> DLGSSQNVNVSSLSGHNYLCPNDWLLNEGKCYWFSTSFKTWKESQRDCTQLQAHLLVIQN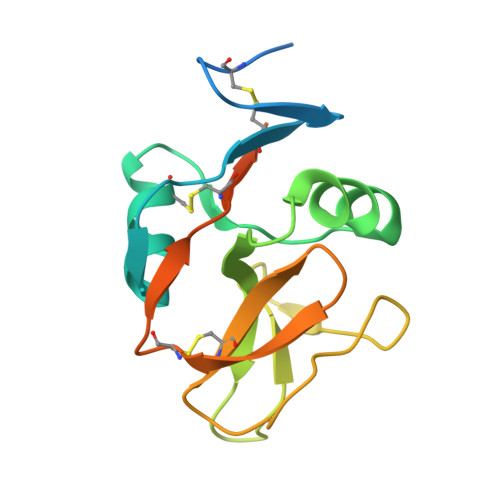LDELEFIQNSLKPGHFGWIGLYVTFQGNLWMWIDEHFLVPELFSVIGPTDDRSCAVITGNWVYSEDCSSTFKGICQRDAILTHNGTSGVAAAHHHHHH> MRGSHHHHHHTDPQGDAAQKTDTSHHDQDHPTFNKITPNLAEFAFSLYRQLAHQSNSTNIFFSPVSIATAFAMLSLGTKADTHDEILEGLNFNLTEIPEAQIHEGFQELLRTLNQPDSQLQLTFGNGLFLSEGLKLVDKFLEDVKKLYHSEAFTVNFGDTEEAKKQINDYVEKGTQGKIVDLVKELDRDTVFALVNYIFFKGKWE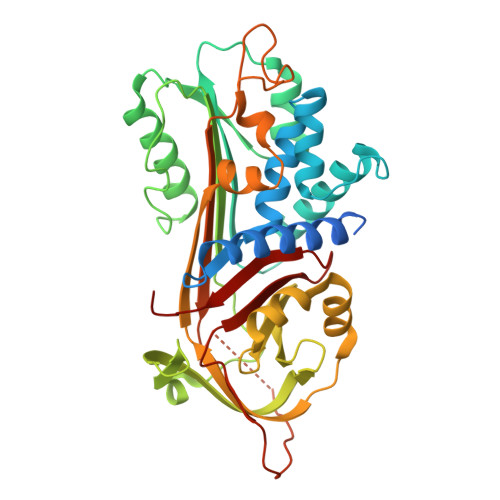RPFEVKDTEEEDFHVDQVTTVKVPMMKRLGMFNIQHCKKLSSWVLLMKYLGNATAIFFLPDEGKLQHLENELTHDIITKFLENEDRRSASLHLPKLSITGTYDLKSVLGQLGITKVFSNGADLSGVTEEAPLKLSKAVHKAVLTIDEKGTEAAGAMFLEAIPMSIPPEVKFNKPFVFLMIEQNTKSPLFMGKVVNPTQK> MKLERVTVKNFRSHSDTVVEFKEGINLIIGQNGSG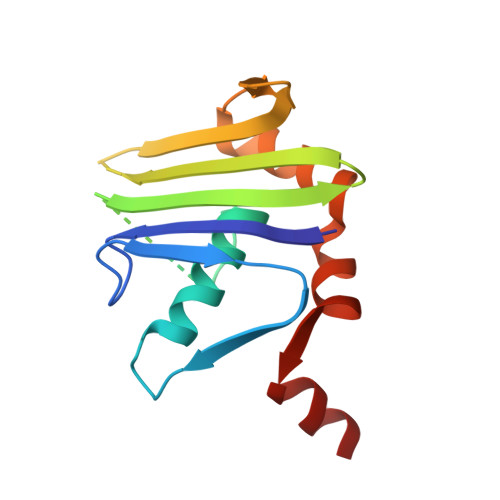KSSLLDAILVGLYWPLRIKDIKKDEFTKVGARDTYIDLIFEKDGTKYRITRRFLKGYSSGEIHAMKRLVGNEWKHVTEPSSKAISAFMEKLIPYNIFLNAIYIRQGQIDAIL> ECGWRIGEAGTDPNLNHQQFRAKILSIW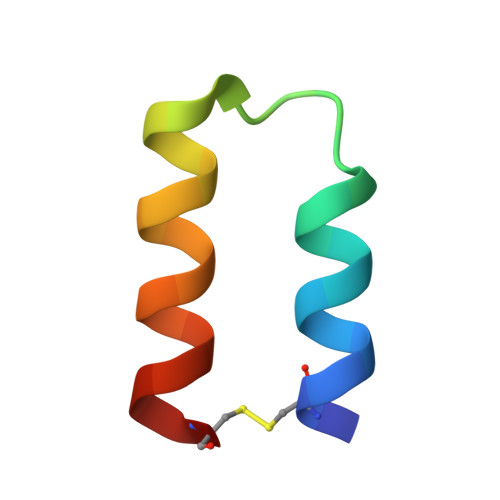EECX5-azanyl-2-[(3~{S})-2,5-bis(oxidanylidene)pyrrolidin-3-yl]isoindole-1,3-dione | C12 H9 N3 O4 | 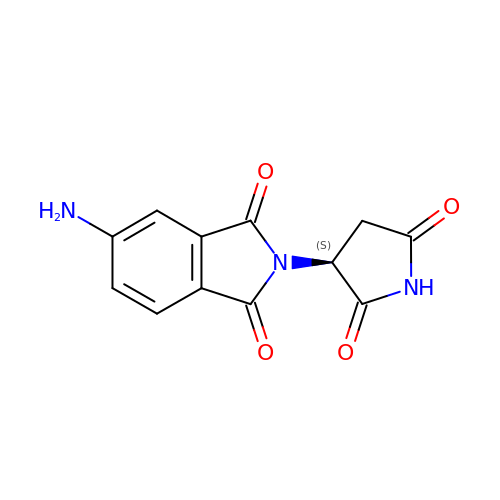ZQAUOFWDVHCTPN-QMMMGPOBSA-N>[6x]LTAKHRPSVVWLHNAECTGCTEAAIRTIKPYIDALILDTISLDYQETIMAAAGEAAEAALHQALEGKDGYYLVVEGGLPTIDGGQWGMVAGHPMIETTKKAAAKAKGIICIGTCSAYGGVQKAKPNPSQAKGVSEALGVKTINIPGCPPNPINFVGAVVHVLTKGIPDLDENGRPKLFYGELVHDNCPRLPHFEASEFAPSFDSEEAKKGFCLYELGCKGPVTYNNCPKVLFNQVNWPVQAGHPCLGCSEPDFWDTMTPFYEQG;>[6x]ASWSHPQFEKGASGAAESKPTPQSTFTGPIVVDPITRIEGHLRIMVEVENGKVKDAWSSSQLFRGLEIILKGRDPRDAQHFTQRACGCCTYVHALASSRCVDDAVKV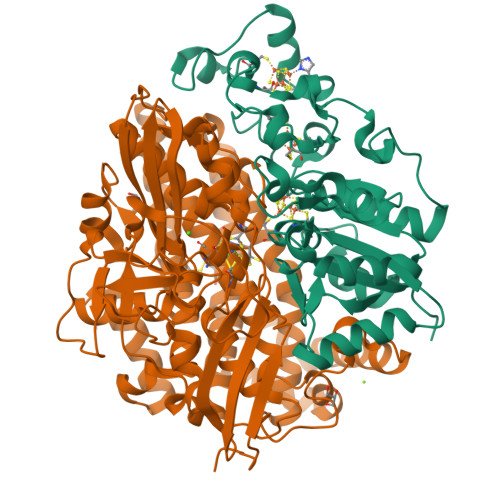SIPANARMMRNLVMASQYLHDHLVHFYHLHALDWVDVTAALKADPNKAAKLAASIAPARPGNSAKALKAVQDKLKAFVESGQLGIFTNAYFLGGHKAYYLPPEVDLIATAHYLEALHMQVKAASAMAILGGKNPHTQFTVVGGCSNYQGLTKDPLANYLALSKEVCQFVNECYIPDLLAVAGFYKDWGGIGGTSNYLAFGEFATDDSSPEKHLATSQFPSGVITGRDLGKVDNVDLGAIYEDVKYSWYAPGGDGKHPYDGVTDPKYTKLDDKDHYSWMKAPRYKGKAMEVGPLARTFIAYAKGQPDFKKVVDMVLGKLSVPATALHSTLGRTAARGIETAIVCANMEKWIKEMADSGAKDNTLCAKWEMPEESKGVGLADAPRGALSHWIRIKGKKIDNFQLVVPSTWNLGPRGAQGDKSPVEEALIGTPIADPKRPVEILRTVHAFDPCIACGVH> GHMNVKLKVFHAGSLTEPMKA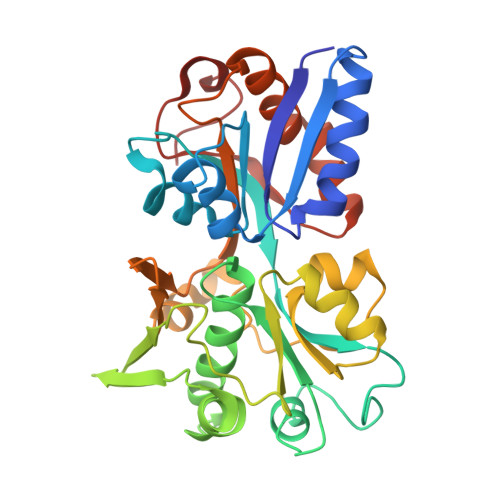FKRAFEEKHPNVEVQTEAAGSAATIRKVTELGRKADVIATADYTLIQKMMYPEFANWTIMFAKNQIVLAYRNDSRYADEINSQNWYEILKRPDVRFGFSNPNDDPCGYRSLMAIQLAELYYNDPTIFDELVAKNSNLRFSEDNGSYVLRMPSSERIEINKSKIMIRSMEMELIHLVESGELDYFFIYKSVAKQHGFNFVELPVEIDLSSPDYAELYSKVKVVLANGKEVTGKPIVYGITIPKNAENRELAVEFVKLVISEEGQEILRELGQEPLVPPRADTAVPSLKAMVEVS Beta-Myrcene | C10 H18 | 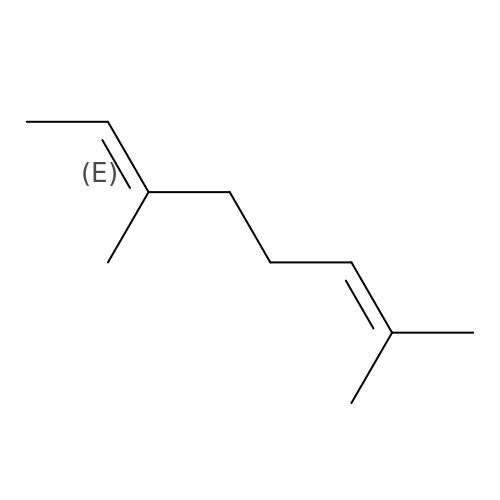MZPDTOMKQCMETI-BJMVGYQFSA-N>[2x]MAHHHHHHVGTFENITAAPADPILGLADLFRADERPGKINLGIGLYYDETGKIPVLTSVKKAEQYLLENETTKLYLGIDGIPEFGRCTQELLFGKGSALINDKRARTAQTPGGSGALRVAADFLAKNTSVKRVWVSNPSWPNHKSVFNSAGLEVREYAYYDAENHTLDFDALINSLNEAQAGDVVLFHGCCHNPTGIDPTLEQWQTLAQLSVEKGWLPLFDFAYQGFARGLEEDAEGLRAFAAMHKELIVASSYSKNFGLYNERVGACTLVAADSETVDRAFSQMKAAIRANYSSPPAHGASVVATILSNDALRAIWEQELTDMRQRIQRMRQLFVNTLQEKGANRDFSFIIKQNGMFSFSGLTKEQVLRLREEFGVYAVASGRVNVAGMTPDNMAPLCEAIVAVL

E. coli aspartate aminotransferase (AAT) is a pyridoxal phosphate (PLP)-dependent enzyme that catalyses the reversible transamination of l-aspartate with α-ketoglutarate, yielding oxaloacetate and l-glutamate. During its catalytic cycle, AAT undergoes hinge movement to switch between an open conformation, in the ligand-free form, and a closed conformation upon association with substrates or inhibitors. Using our approach, we enrich the less populated but catalytically active closed conformation in order to increase catalytic efficiency (kcat/KM) with the non-native substrate l-phenylalanine, leading to altered substrate selectivity. Steady-state kinetics reveal kcat/KM increases of up to 100-fold towards this aromatic amino acid, resulting in a selectivity switch of up to 1900-fold, and structural analyses by room-temperature X-ray crystallography and multitemperature nuclear magnetic resonance (NMR) spectroscopy confirm that the conformational landscape is remodeled to favor the target state.

To obtain structures in the absence of maleate, we applied a rigorous crystal soaking method to serially dilute and extract the inhibitor from the crystallized enzymes. Overlay of AAT structures (Chain A) in the presence and absence of maleate show transition from open to closed states upon inhibitor binding for WT, VFCS, and AIFS, but not for HEX, VFIT, and VFIY, which already adopt the closed conformation in the absence of bound inhibitor. Superposition of bound and unbound structures for each variant confirmed that closed library mutants VFIT and VFIY remained in the closed conformation in the inhibitor-free form, similar to HEX, while OpenLow variant VFCS and OpenHigh variant AIFS adopted the open conformation, similar to WT. By contrast, the HEX spectrum at 278 K showed a large broad peak centered at around ‒61.6 ppm, with another peak of substantially lower intensity also appearing at a similar shift to that observed in the WT spectrum (‒60.4 ppm). We calculated ΔG at 278 K for HEX to be –1.72 kcal mol–1, a small difference that would be compatible with the interconversion between these two states to be part of the catalytic cycle.>MKLPVREFDAVVIGAGGAGMRAALQISQSGQTCALLSKVFPTRSHTVSAQGGITVALGNTHEDNWEWHMYDTVKGSDYIGDQDAIEYMCKTGPEAILELEHMGLPFSRLDDGRIYQRPFGGQSKNFGGEQAARTAAAADRTGHALLHTLYQQNLKNHTTIFSEWYALDLVKNQDGAVVGCTALCIETGEVVYFKARATVLATGGAGRIYQSTTNAHINTGDGVGMAIRAGVPVQDMEMWQFHPTGIAGAGVLVTEGCRGEGGYLLNKHGERFMERYAPNAKDLAGRDVVARSIMIEIREGRGCDGPWGPHAKLKLDHLGKEVLESRLPGILELSRTFAHVDPVKEPIPVIPTCHYMMGGIPTKVTGQALTVNEKGEDVVVPGLFAVGEIACVSVHGANRLGGNSLLDLVVFGRAAGLHLQESIAEQGALRDASESDVEASLDRLNR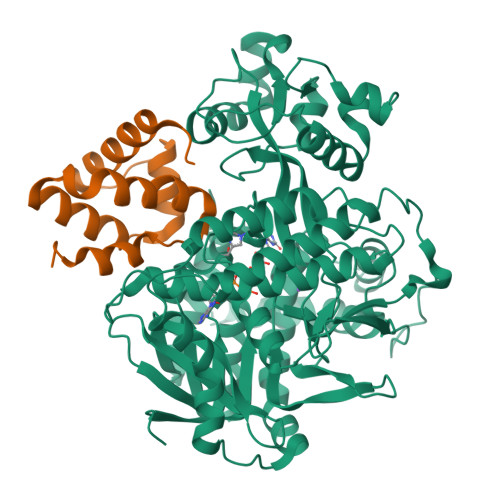WNNNRNGEDPVAIRKALQECMQHNFSVFREGDAMAKGLEQLKVIRERLKNARLDDTSSEFNTQRVECLELDNLMETAYATAVSANFRTESRGAHSRFDFPDRDDENWLCHSLYLPESESMTRRSVNMEPKLRPAFPPKIRTY[2x];>[2x]MGSSHHHHHHSQDPDINNKARIHWACRRGMRELDISIMPFFEHEYDSLSDDEKRIFIRLLECDDPDLFNWLMNHGKPADAELEMMVRLIQTRNRERGPVAI>[5x]QPALLRLSDHLLANYKKGVRPVRDWRKPTTVSIDVIMYAILNVDEKNQVLTTYIWYRQYWTDEFLQWTPEDFDNVTKLSIPTDSIWVPDILINEFVDVGKSPNIPYVYVHHRGEVQNYKPLQLVTACSLDIYNFPFDV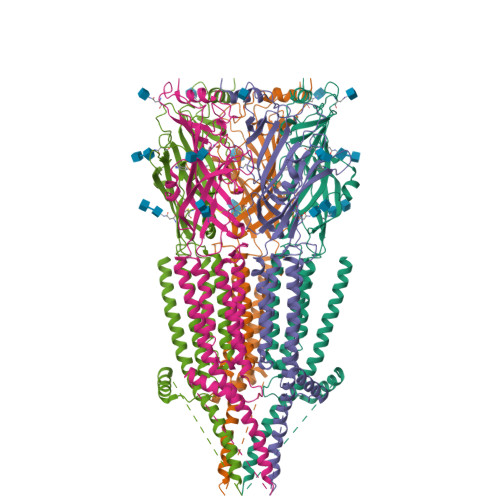QNCSLTFTSWLHTIQDINITLWRSPEEVRSDKSIFINQGEWELLEVFPQFKEFSIDISNSYAEMKFYVIIRRRPLFYAVSLLLPSIFLMVVDIVGFCLPPDSGERVSFKITLLLGYSVFLIIVSDTLPATAIGTPLIGVYFVVCMALLVISLAETIFIVRLVHKQDLQRPVPDWLRHLVLDRIAWILCLGEQPMAHRPPATFQANKTDDCSGSDLLPAMGNHCSHVGGPQDLEKTPRGRGSPLPPPREASLAVRGLLQELSSIRHFLEKRDEMREVARDWLRVGYVLDRLLFRIYLLAVLAYSITLVTLWSIAW>MSSGSRRGGNVYREPGSAAADLFERARRVLPGGNTRTTVYSAPYPPYAARGRGAVIVDADGEERLDFVNNYTALIHGHADPDINEAVIRQLADGVAFAMPTEHEIALAELLTERVPSLQQVRFTNSGTEAVMMAIKAARAYTGRPRIAKFDGCYHGSYDFAEVSTQSSGKPGEDGFPVATPYTGGTPQAVLDSVVVLPFNDIDGTERLIEQHRDELAAVLIDPNPRSLGLYPAEPAFLQRLREITRAYGIVLIFDEVISLRSDYGGMQSVLGVTPDLTAMGKIIGGGFPVGAVGGSAE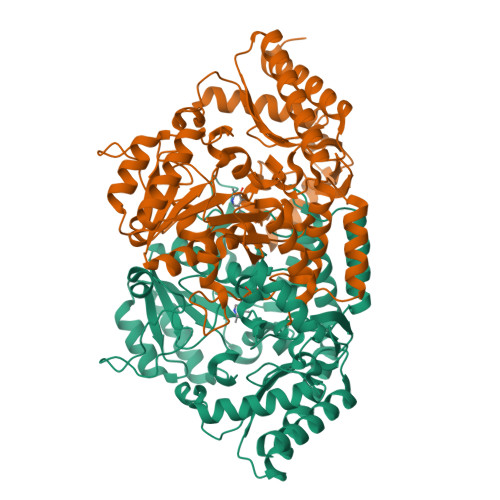VMSVFDPTGGPPRAPHGGTFNANPVTMVAGLTAMRKLTPAEFDRLATLGQQLRAGVEEVLREAGVPGQVTGYGSLFHIHLHQRPLADYRNSVLSAQERAFVGRVHEALMGRGIFITPALFGCLSTPMGVPEVEAFVDAFAAALQDARGLEHHHHHH[2x]>[2x]GSITENTSWNKEFSAEAVNGVFVLCKSSSKSCATNDLARASKEYLPASTFKIPNAIIGLETGVIKNEHQVFKWDGKPRAMKQWERDLTLRGAIQVSAVPVFQQIAREVGEV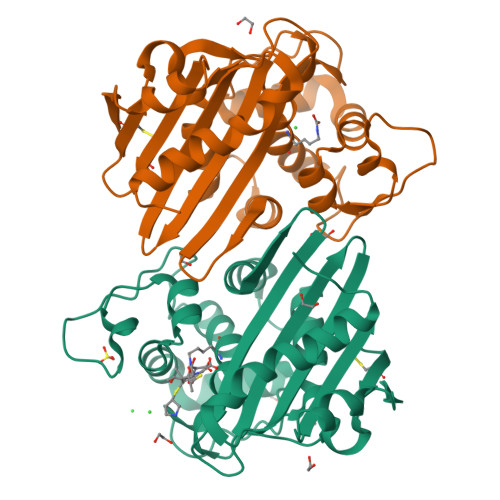RMQKYLKKFSYGNQNISGGIDKFWLEGQLRISAVNQVEFLESLYLNKLSASKENQLIVKEALVTEAAPEYLVHSKTGYSTRIEPKIGWWVGWVEKETEVYFFAFNMDIDNESKLPLRKSIPTKIMESEGIIGG>[2x]KPTVKEIKSLQNFNRIAGVFHLLQMLAVLALANDFALPMTGTYLNGPPGTTFSAPVVILETPVGLAVALFLGLSALFHFIVSSGNFFKRYSASLMKNQNIFRWVEYSLSSSVMIVLIAQICGIADIVALLAIFGVNASMILFGWLQEKYTQPKDGDLLPFWFGCIAGIVPWIGLLIYVIAPGSTSDVAVPGFVYGIIISLFLFFNSFALVQYLQYKGKGKWSNYLRGERAYIVLSLVAKSALAWQIFSGTLI

Heliorhodopsins (HeRs) are a new class of Microbial rhodopsins (MRs), with a low homology (<15%) to all other MRs and a unique membrane topology in which their N-termini face the intracellular side and C-termini face the extracellular side. To explore the photoactivation mechanism of HeRs, we sought to solve the structure of HeR 48C12 (hereafter referred to as HeR). Despite the unique topology and low homology to other MRs, the structure of HeR shows a typical seven transmembrane helix bundle of MRs. Overall, we have reported the novel structure of HeR 48C12 and mechanistically addressed the key physiological properties of HeR, such as pump/channel activity and the long photocycle.

Well-diffracting HeR protein crystals were grown in lipid cubic phase, and the structure was solved at 2.7 Å resolution. The structure contains two HeR molecules in each asymmetric unit (designated as chains A and B) and the two molecules align very well with each other (RMSD = 0.361 Å). The most striking feature of the HeR structure is the very long extracellular loop 1 (ECL1) that is mainly composed of two antiparallel β-strands, which has never been seen in other rhodopsins. The structure also revealed that HeR forms a dimer. The overall dimer interface is 2260 Å2 as calculated by ccp4 program PISA,2 which is the most extensive dimerization interface seen in MRs. Compared to the classic bacterial rhodopsin (BR),3,4 the hydrophobic core architecture for ATR binding is well conserved in HeR; in particular, the π-electron system formed by two aromatic residues (W182/W86 for BR, F206/Y108 for HeR) at both sides of ATR, is critical for stabilizing the protonated polyethylene chain of ATR. Compared to BR, several key residues are missing in the HeR structure. In the Schiff base region, the key residue D212 is changed to S237 in HeR; and most dramatically the key residues for proton release, E204 and E194, are missing in HeR. In contrast, the ‘tunnel’ formed by TM1, 2, 3 and 7 of HeR is filled with hydrophobic residues, e.g., F88, V83, F72, V69 and V65 of TM2, L118 of TM3, and I9 of TM1, which occlude ions from passing through this tunnel. Our structure shows that H23 and H80 are isolated from detectable polar interaction to the proton transferring chain centered at E107.>MGSSHHHHHHSSGRENLYFQGMIYMPIVVAVDKKSDRAERVLRFAAEEARLRGVPVYVVHSLPGGGRTKDEDIIEAKETLSWAVSIIRKEGAEGEEHLLVRGKEPPDDIVDFADEVDAIAIVIGIRKRSPTGKLIFGSVARDVILKA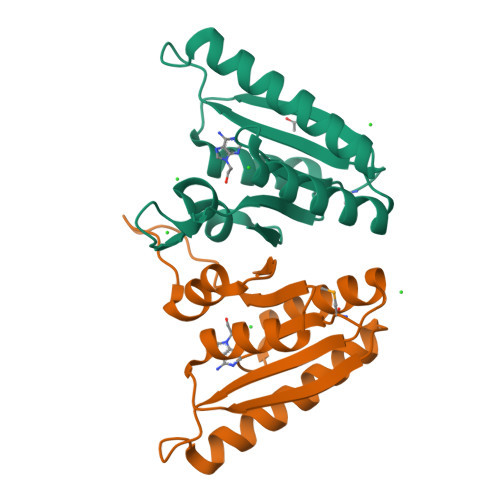NKPVICIK[4x]> MAQQKKTIAVVNATGRQAASLIRVAAAVGHHVRAQVHSLKGLIAEELQAIPNVTLFQGPLLNNVPLMDTLFEGAHLAFINTTSQAGDEIAIGKDLADAAKRAGTIQHYIYSSMPDHSLYGPWPAVPMWAPKFTVENYVRQLGLPSTFVYAGIYNNNFTSLPYPLFQMELMPDGTFEWHAPFDPDIPLPWLDAEHDVGPALLQIFKDGPQKW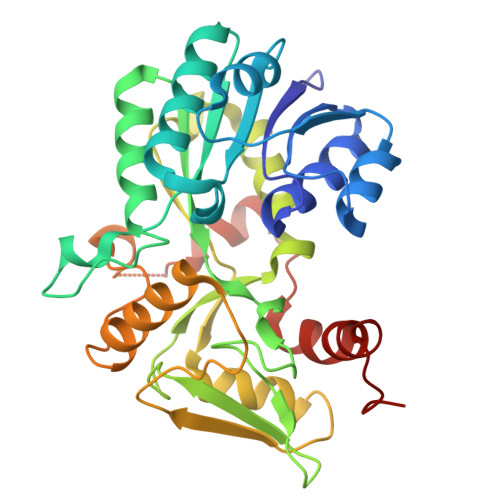NGHRIALTFETLSPVQVCAAFSRALNRRVTYVQVPKVEIKVNIPVGYREQLEAIEVVFGEHKAPYFPLPEFSRPAAGSPKGLGPANGKGAGAGMMQGPGGVISQRVTDEARKLWSGWRDMEEYAREVFPIEEEANGLDWML>[4x]SNA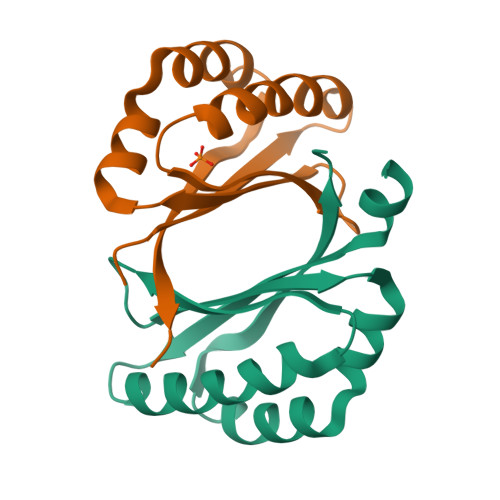MQKIKSEERHIICELRCEPENRERVKELVLKFVEPARLETGCLYYDLYQKIDEPDTFYIIDGWVNQEAVTSHAENPHVAEVMSDLQPLLTFGPSISLITRVSD>DISKLISRGTFDQMLKHRNDGACPAKGFYTYDAFIAAAKAFPGFGTTGDDATRKREIAAFLGQTSHETTGGWPSAPDGPYSWGYCFLREKNPSSSYCSPSPTYPCAPGKQYYGRGPIQLSWNYNYGPCGKA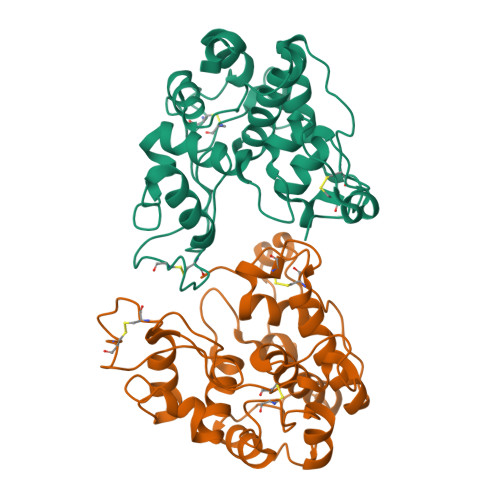IGVDLLNNPDLVATDPVISFKTALWFWMTPQSPKPSCHNVITGIWKPSAADQSAGRVPGYGATTNIINGGLECGQGWKPQVEDRIGFYKRYCDIFKVGYGNNLDCYNQRPFGSG[4x]> MGSDKIHHHHHHMKGVIEYSLKTSNDDQFIDITNLVKKAVDESGVSDGMAVVFCPHTTA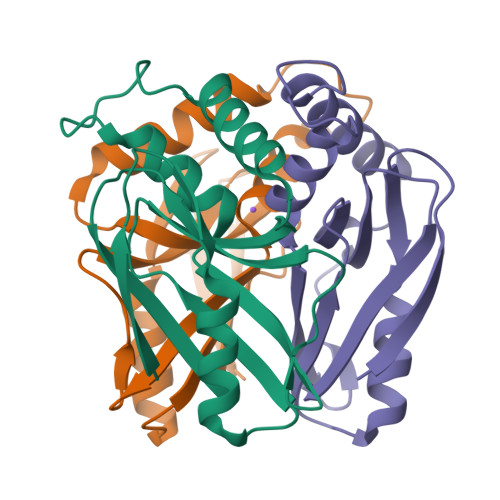GITINENADPDVTRDILVNLDKVFPKVGDYKHVEGNSHAHIKASLMGSSQQIIIENGKLKLGTWQGIYFTEFDGPRDRKVFVKII>[2x]SNAMYTHSKQIITSGVPVQRAKKAVVMLHGRGGTAADIISLQKVLKLDEMAIYAPQATNNSWYPYSFMAPVQQNQPALDSALALVGEVVAEIEAQGIPAEQIYFAGFSQGACLT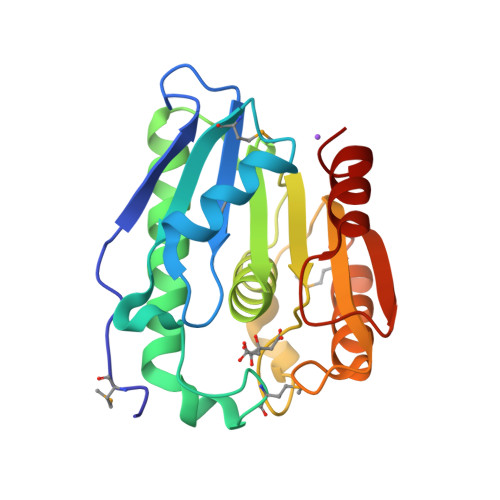LEYTTRNARKYGGIIAFTGGLIGQELAIGNYKGDFKQTPVFISTGNPDPHVPVSRVQESVTILEDMNAAVSQVVYPGRPHTISGDEIQLVNNTILK> ENLYFQSMSVKGRIYSILKQIGSGGSSKVFQVLNEKKQIYAIKYVNLEEADNQTLDSYRNEIAYLNKLQQHSDKIIRLYDYEITDQYIYMVMEYGNIDLNSWLKKKKSIDPWERKSYWKNMLEAVHTIHQHGIVHSDLKPANFLIVDGMLKLIDFGIANQMQPDTTSVVKDSQVGTVNYMPPEAIKDMSSSRENG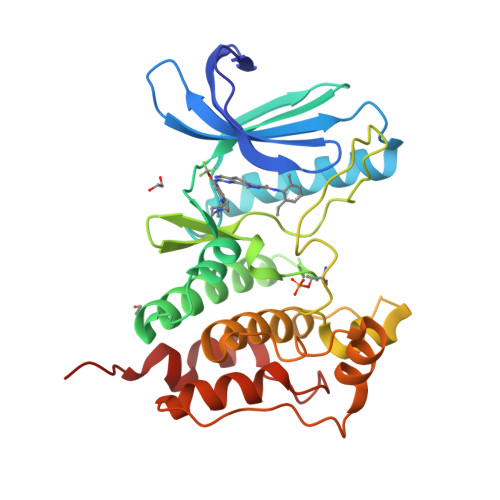KSKSKISPKSDVWSLGCILYYMTYGKTPFQQIINQISKLHAIIDPNHEIEFPDIPEKDLQDVLKCCLKRDPKQRISIPELLAHPYVQIQTHP> MEPFRNIGIIGRLGSTQVLDTIRRLKKFLIDRHLHVILEDTIAEVLPGHGLQTCSRKIMGEICDLVVVVGGDGSMLGAARALARHKVPVLGINRGSLGFLTDIRPDELEAKVGEVLDGQYIVESRFLLDAQVRRGIDSMGQGDALNDVVLHPGKST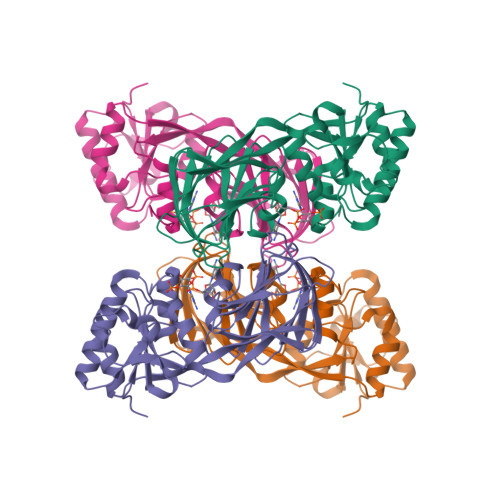RMIEFELYIDGQFVCSQKADGLIVATPTGSTAYALSAGGPIMHPKLDAIVIVPMYPHMLSSRPIVVDGNSELKIVVSPNMQIYPQVSCDGQNHFTCAPGDTVTISKKPQKLRLIHPIDHNYYEICRTKLGWGSRLGGGD> GLPRHSAVMERLRRRIELCRRHHSTCEARYEAVSPERLELERQH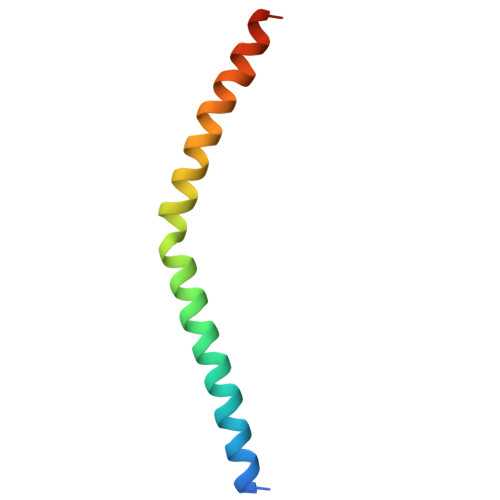TFALHQRCIQAKAKRAGKH> MGVVEEAHNVKVIGSG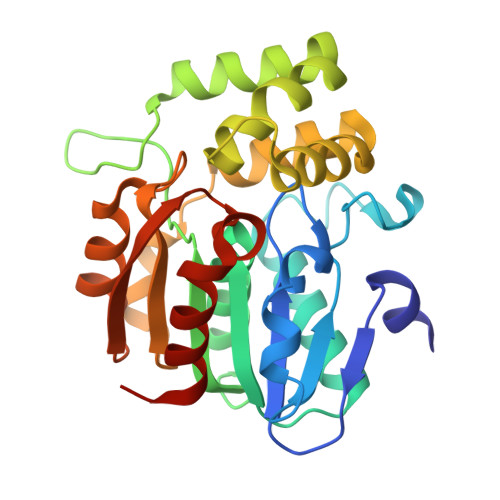EATIVLGHGFGTDQSVWKHLVPHLVDDYRVVLYDNMGAGTTNPDYFDFDRYSNLEGYSFDLIAILEDLKIESCIFVGHSVSAMIGVLASLNRPDLFSKIVMISASPRYVNDVDYQGGFEQEDLNQLFEAIRSNYKAWCLGFAPLAVGGDMDSIAVQEFSRTLFNMRPDIALSVGQTIFQSDMRQILPFVTVPCHILQSVKDLAVPVVVSEYLHANLGCESVVEVIPSDGHLPQLSSPDSVIPVILRHIRNDIAM>SSSSTASASAKKIIVKHVTVIGGGLMGAGIAQVAAATGHTVVLVDQTEDILAKSKKGIEESLRKVAKKKFAENPKAGDECVEKTLSTIATSTDAASVVHSTDLVVEAIVENLKVKNELFKRLDKFAAEHTIFASNTSSLQITSIANATTRQDRFAGLHFFNPVPVMKLVEVIKTPMTSQKTFESLVDFSKALGKHPVSCKDTPGFIVNRLLVPYLMEAIRLYER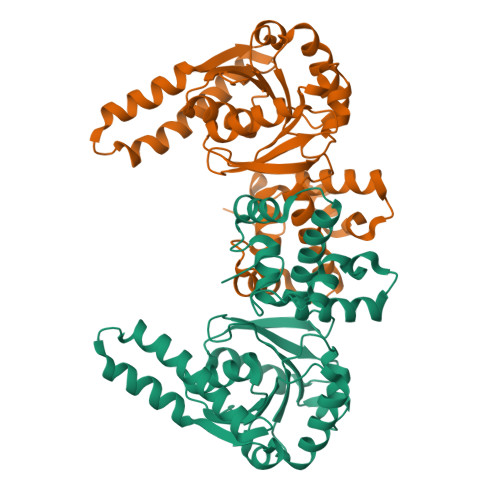GDASKEDIDTAMKLGAGYPMGPFELLDYVGLDTTKFIVDGWHEMDAENPLHQPSPSLNKLVAENKFGKKTGEGFYKYKLEHHHHHH[2x]selinexor, bound form | C17 H13 F6 N7 O | 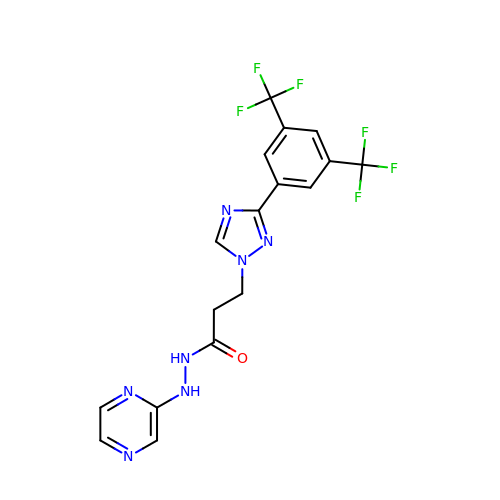SRMSVLNNUIPUGA-UHFFFAOYSA-N>SFTMTWLPLNPIPLKDRVSMIFLQYGQIDVIDGAFVLIDKTGIRTHIPVGSVACIMLEPGTRVSHAAVRLAAQVGTLLVWVGEAGVRVYASGQPGGARSDKLLYQAKLALDEDLRLKVVRKMFELRFGEPAPARRSVEQLRGIEGSRVRATYALLAKQYGVTWNGRRYDPKDWEKGDTINQCISAATSCLYGVTEAAILAAGYAPAIGFVHTGKPLSFVYDIADIIKFDTVVPKAFEIARRNPGEPDREVRLACRDIFRSSKTLAKLIPLIEDVLAAGEIQPPAPPEDAQPVAIPLPVSLGDAGHRSS[4x];>[2x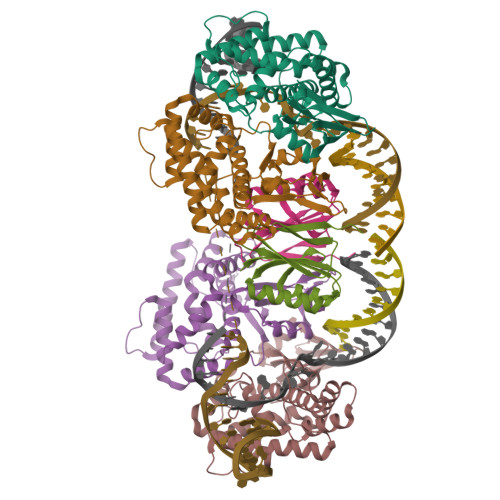]MSMLVVVTENVPPRLRGRLAIWLLEVRAGVYVGDVSAKIREMIWEQIAGLAEEGNVVMAWATNTETGFEFQTFGLNRRTPVDLDGLRLVSFLPV> MHHHHHHENLYFQGQHAQPPPQPRKKRPEDFKFGKILGEGSFSTVVLARELATSREYAIKILEKRHIIKENKVPYVTRERDVMSRLDHPFFVKLYFTFQDDEKLYFGLSYAKNGELLKYIRKIGSFDETCTRFYTAEIVSALEYLHGKGIIHRDLKPENILLNEDMHIQITDFGTAKVLSPESKQARANSFVGTAQYVSPELLTEKSACKSSDLWALGCIIYQLVAGLPPFRAGNEYLIFQKIIKLEYDFPEKFFPKARDLV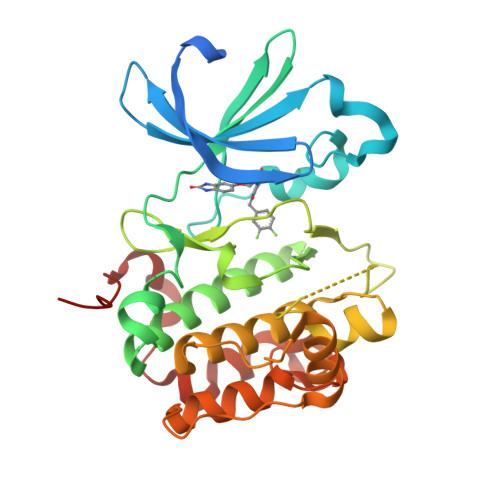EKLLVLDATKRLGCEEMEGYGPLKAHPFFESVTWENLHQQTPPKLTAYL>[2x]MASVNPEYFSAADVYVPDEWEVAREKITMSRELGQGS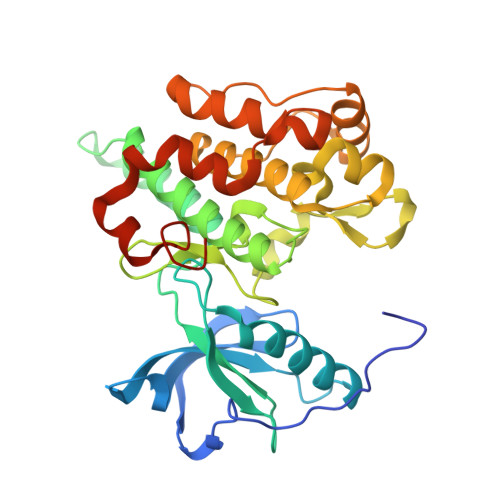FGMVYEGVAKGVVKDEPETRVAIKTVNEAASMRERIEFLNEASVMKEFNCHHVVRLLGVVSQGQPTLVIMELMTRGDLKSYLRSLRPAMANNPVLAPPSLSKMIQMAGEIADGMAYLNANKFVHRDLAARNCMVAEDFTVKIGDFGMTRDIYETDYYRKGGKGLLPVRWMSPESLKDGVFTTYSDVWSFGVVLWEIATLAEQPYQGLSNEQVLRFVMEGGLLDKPDNCPDMLFELMRMCWQYNPKMRPSFLEIISSIKEEMEPGFREVSFYYSEENKLPEPEELD> MSVGKPLPHDSARAHVTGQARYLDDLPCPANTLHLAFGLSTEASAAITGLDLEPVRESPGVIAVFTAADLPHDNDASPAPSPEPVLATGEVHFVGQPIFLVAATSHRAARIAARKARITYAPRPAILTLDQALAADSRFEGGPVIWARGDVETALAGAAHLAEGCFEIGGQEHFYLEGQAALALPAEGGVVIHCSS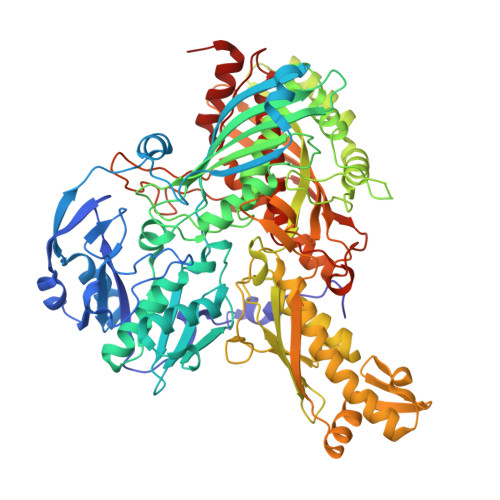QHPSEIQHKVAHALGLAFHDVRVEMRRMGGGFGGKQSQGNHLAIACAVAARATGRPCKMRYDRDDDMVITGKRHDFRIRYRIGADASGKLLGADFVHLARCGWSADLSLPVCDRAMLHADGSYFVPALRIESHRLRTNTQSNTAFRGFGGPQGALGMERAIEHLARGMGRDPAELRALNFYDPPERGGLSAPPSPPEPIATKKTQTTHYGQEVADCVLGELVTRLQKSANFTTRRAEIAAWNSTNRTLARGIALSPVKFGISFTLTHLNQAGALVQIYTDGSVALNHGGTEMGQGLHAKMVQVAAAVLGIDPVQVRITATDTSKVPNTSATAASSGADMNGMAVKDACETLRGRLAGFVAAREGCAARDVIFDAGQVQASGKSWRFAEIVAAAYMARISLSATGFYATPKLSWDRLRGQGRPFLYFAYGAAITEVVIDRLTGENRILRTDILHDAGASLNPALDIGQIEGAYVQGAGWLTTEELVWDHCGRLMTHAPSTYKIPAFSDRPRIFNVALWDQPNREETIFRSKAVGEPPFLLGISAFLALHDACAACGPHWPDLQAPATPEAVLAAVRRAEGRA> GSHMTALDWRSALTADEQRSVRALVTATTAVDGVAPVGEQVLRELGQQRTEHLLVAGSRPGGPIIGYLNLSPPRGAGGAMAELVVHPQSRRRGIGTAMARAALAKTAGRNQFWAHGTLDPARATASALGLVGVRELIQMRRPLRDIPEPTIPDGVVIRTYAGTSDDAELLRVNNAAFAGHPEQGGWTAVQLAERRGEAWFDPDGLILAFGDSPRERPGRLLGFHWTKVHPDHPGLGEVYVLGVDPAAQRRGLGQMLTSIGIVSLARRLGG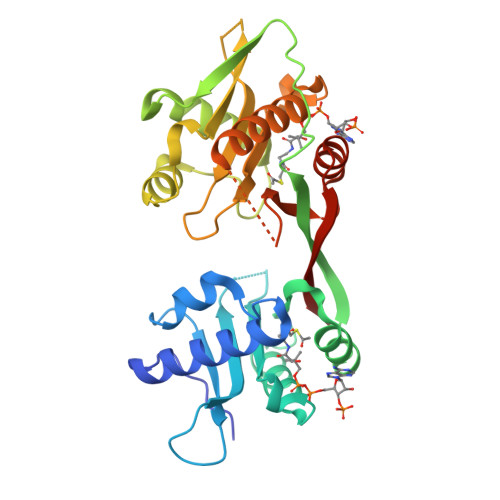RKTLDPAVEPAVLLYVESDNVAAVRTYQSLGFTTYSVDTAYALAGTDN>[2x]HMGSEAAQLLEAADFAARKHRQQRRKDPEGTPYINHPIGVARILTHEAGITDIVVLQAALLHDTVEKTDTTLDEVELHF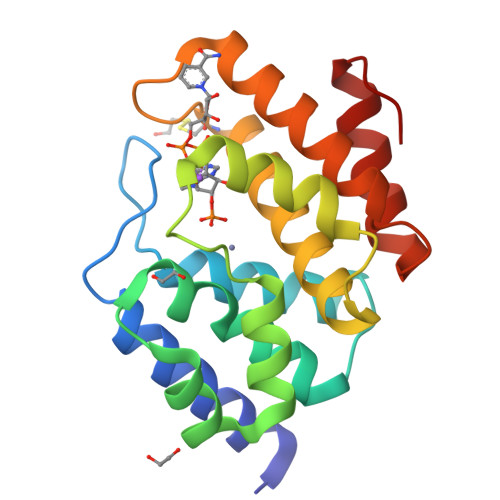GAQVRRLVEEVTDDKTLPKLERKRLQVEQAPHSSPGAKLVKLADKLYNLRDLNRCTPEGWSEHRVQEYFEWAAQVVKGLQGTNRQLEEALKHLFKQRGLTI>[5x]VPQKPKVSLNPPWNRIFKGENVTLTCNGNNFFEVSSTKWFHNGSLSEETNSSLNIVNAKFEDSGEYKCQHQQVNESEPVYLEVFSDWL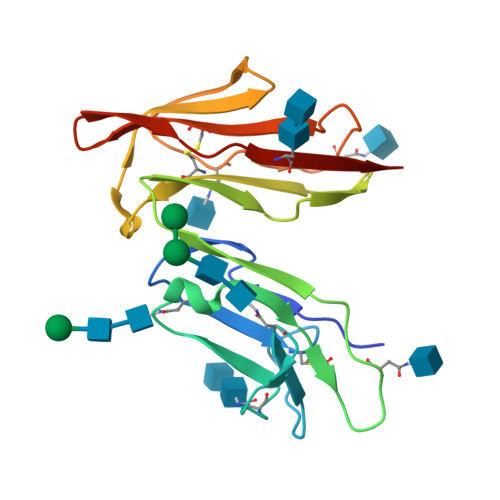LLQASAEVVMEGQPLFLRCHGWRNWDVYKVIYYKDGEALKYWYENHNISITNATVEDSGTYYCTGKVWQLDYESEPLNITVIKA> MILDTDYITEDGKPVIRIFKKENGEFKIEYDRTFEPYFYALLKDDSAIEEVKKITAERHGTVVTVKRVEKVQKKFLGRPVEVWKLYFTHPQDVPAIRDKIREHPAVIDIYEYDIPFAKRYLIDKGLVPMEGDEELKMLAFDIETLYHEGEEFAEGPILMISYADEEGARVITWKNVDLPYVDVVSTEREMIKRFLRVVKEKDPDVLITYNGDNFDFAYLKKRCEKLGINFALGRDGSEPKIQRMGDRFAVEVKGRIHFDLYPVIRRTINLPTYTLEAVYEAVFGQPKEKVYAEEITTAWETGENLERVARYSMEDAKVTYELGKEFLPMEAQLSRLIGQSLWDVSRSSTGNLVEWFLLRKAYERNELAPNKPDEKELARRRQSYEGGYVKEPERGLWENIVYLDFRSLYPSIIITHNVSPDTLNREGCKEYDVAPQVGHRFCKDFPGFIPSLLGDLLEERQKIKKKMKATIDPIERKLLDYRQRRIKILASSYYGYYGYARARWYCKECAESVTAWGREYITMTIKEIEEKYGFKVIYSDTDGFFATIPGADAETVKKKAMEFLKYINAKLPGALELEYEGFYKRGFFVTKKKYAVIDEEGKITTGGLEIVRRDWSEIAKETQARVLEALLKDGDVEKAVRIVKEVTEKLSKYEVPPEKLVIHEQITRDLKDYKATGPHVAVAKRLAARGVKIRPGTVISYIVLKGSGRIGDRAIPFDEFDPAKHKYDAEYYIENQVLPAVERILRAFGYRKEDLRYQKTRQVGLSAWLKPKGT

Kod-RI is an engineered TNA polymerase that was evolved from a replicative B-family DNA polymerase isolated from the archaeal hyperthermophilic species Thermococcus kodakarensis (Kod). The polymerase harbors the A485R and E664I mutations required for TNA synthesis on DNA templates, as well as the 3′,5′-exonuclease silencing mutations (D141A, E143A) that prevent the removal of newly added TNA residues. Phosphonomethylthreosyl nucleic acid (pTNA, also abbreviated PMT and tPhoNA) is considered a possible XNA candidate for information storage in cellular systems. pTNA is an unusual example of an XNA; it contains modifications in both the sugar and phosphodiester moieties with α-l-threofuranosyl sugars connected by 3′→2′ phosphonomethyl backbone linkages. X-ray crystal structures of the post-catalytic complex showing Kod-RI bound to a DNA substrate that had been extended with either two pTNA adenosine residues (ptA) or two 2′-deoxyadenosine residues (dA) were solved to high resolution.

Kod-RSGA is a more efficient TNA polymerase that was recently discovered by programmed allelic mutagenesis. Similar to Kod-RI, Kod-RSGA contains the exonuclease silencing mutations (D141A and E143A) and shares the A485R gain-of-function mutation necessary for TNA synthesis. Additional mutations include N491S located in the finger subdomain, as well as the mutations R606G and T723A, both of which are located in the thumb subdomain. Primer extension assays comparing Kod-RI and Kod-RSGA as polymerases for pTNA synthesis on a DNA template reveal that Kod-RSGA functions with higher overall activity than Kod-RI. To better understand the activity of Kod-RSGA as a pTNA polymerase, we solved the X-ray crystal structure of Kod-RSGA in the post-catalytic state following two cycles of pTNA addition to the 3′-end of the DNA primer. The structure resolved to a resolution of 3.01 Å, enabling a detailed comparison with the equivalent structure of Kod-RI TNA polymerase. The conformation of the pTNA nucleotides in Kod-RSGA strongly resembles the conformation of pTNA in Kod-RI in terms of torsion angles of the backbone and sugar pucker. The biggest difference between the Kod-RI and Kod-RSGA structures extended with pTNA is the structural rearrangement observed as a result of the R606G mutation found in Kod-RSGA. In Kod-RSGA, this position is mutated to a glycine residue, which allows Y594 to form a strong hydrogen bond to the same phosphate group previously contacted by the R606. We postulate that this interaction may also be important for pTNA synthesis, since Kod-RSGA is a more efficient pTNA polymerase than Kod-RI.> MSKSIYEQYLQAKADNPGKYARDLATLMGISEAELTHSRVSHDAKRLKGDARALLAALEAVGEVKAITRNTYAVHEQMGRYENQHLNGHAGLILNPRNLDLRLFLNQWASAFTLTEETRHGVRHSIQFFDHQGDALHKVYVTEQTDMPAWEALLAQFITTENPE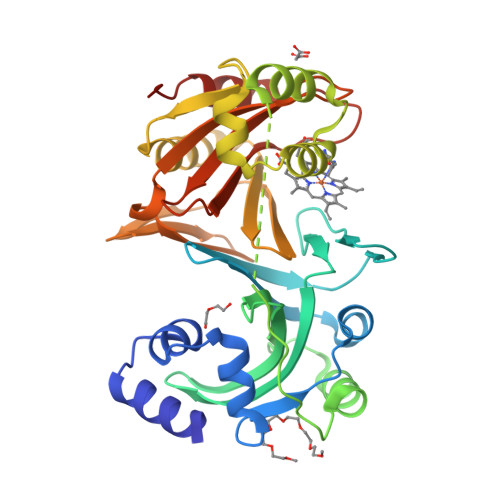LQLEPLSAPEVTEPTATDEAVDAEWRAMTDVHEFFQLLKRNNLTRQQAFRAVGNDLAYQVDNSSLTQLLNIAQQEQNEIMIFVGNRGCVQIFTGMIEKVTPHQDWINVFNQRFTLHLIETTIAESWITRKPTKDGFVTSLELFAADGTQIAQLYGQRTEGQPEQTQWRDQIARLNNKDIAA> HSFLVDASPSAKDHVAASPKLVKLRFGGGVEPAYSSISILDSTGKLVVEGAKGQADKPRELTLDAPELAVGS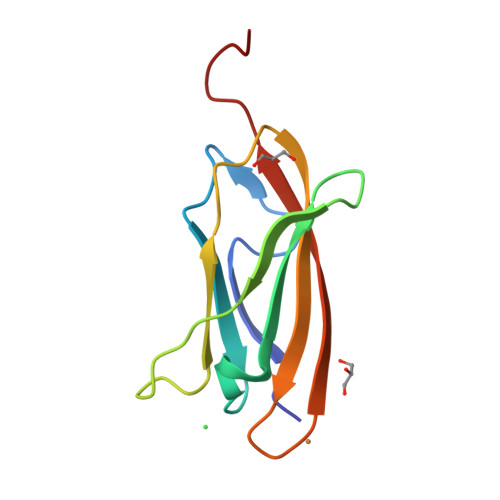YVVKFRVLSSDGHIVEGKYEFTVDPHENLY>[2x]MD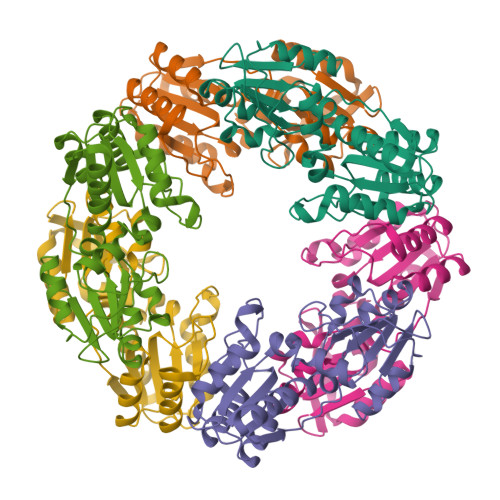RDELVRYLDAYLRIQDFPQDPSLNGLQVEGKRTVRKVGAAVDAGEAIFRKALEEEVDFLIVHHGLFWGKPFPIVGHHKRRLETLFQGGINLYAAHLPLDAHEEVGNNFVLARELGLVDLTPWDVGVKGRFPQPTPLLQVADRLGQLTGMQPLVHQGGLDHVETVILVSGSGTGLLPKVDADLFVTGEPKHSVFHETFERGLNVIYAGHYDTETFGVKALAAHLEARFGLPWVFLDHPTGL> ENLTPQHMASMALTGTDRVKRGMAEMQKGGVIMDVVNAEQAKIAEAAGAVAVMALERVPADIRAAGGVAR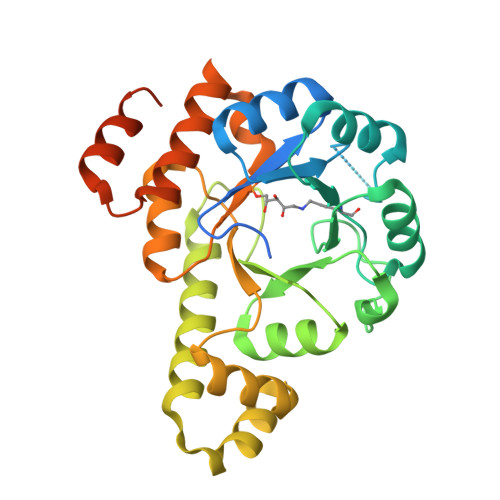MADPTVIEEVMNAVSIPVMAXVRIGHYVEARVLEALGVDYIDESEVLTPADEEFHIDKRQFTVPFVCGCRDLGEAARRIAEGASMLRTKGEPGTGNIVEAVRHMRKVNAQIRKVVNMSEDELVAEAKQLGAPVEVLREIKRLGRLPVVNFAAGGVTTPADAALMMHLGADGVFVGSGIFKSENPEKYARAIVEATTHYEDYELIAHLSKGLGGAMRGIDIATLLPEHRMQERGWA>RADPDPMKNTCKLLVVADHRFYRYMGRGEESTTTNYLIELIDRVDDIYRNTAWDNAGFKGYGIQIEQIRILKSPQEVKPGEKHYNMAKSYPNEEKDAWDVKMLLEQFSFDIAEEASK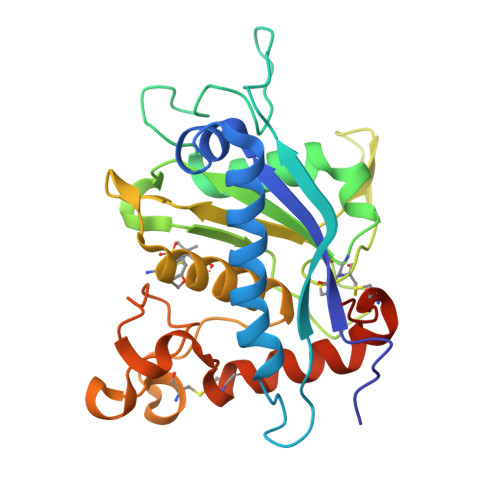VCLAHLFTYQDFDMGTLGLAYVGSPRANSHGGVCPKAYYSPVGKKNIYLNSGLTSTKNYGKTILTKEADLVTTHELGHNFGAEHDPDGLAECAPNEDQGGKYVMYPIAVSGDHENNKMFSQCSKQSIYKTIESKAQECFQERSNKVGSHHHHHH[2x]> GPMAGAATQASLESAPRIMRLVAECSRSRARAGELWLPHGTVATPVFMPVGTQATMKGITTEQLDALGCRICLGNTYHLGLRPGPELIQKANGLHGFMNWPHNLLTDSGGFQMVSLVSLSEVTEEGVRFRSPYDGNETLLSPEKSVQIQNALGSDIIMQLDDVVSSTVTG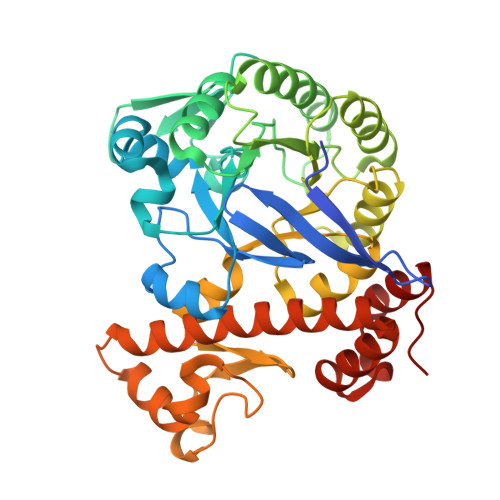PRVEEAMYRSIRWLDRCIAAHQRPDKQNLFAIIQGGLDADLRATCLEEMTKRDVPGFAIGGLSGGESKSQFWRMVALSTSRLPKDKPRYLMGVGYATDLVVCVALGCDMFDCVFPTRTARFGSALVPTGNLQLRKKVFEKDFGPIDPECTCPTCQKHSRAFLHALLHSDNTAALHHLTVHNIAYQLQLMSAVRTSIVEKRFPDFVRDFMGAMYGDPTLCPTWATDALASVGITLG> DQSDLHISDQTDTKGTVCSPFALFAVLENTGEKLKKSKWKWELHKLENARKPLKDGNVIEKG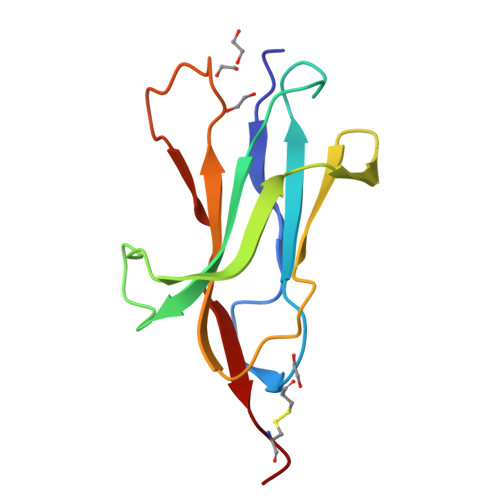FVSNQIGDSLYKIETKKKMKPGIYAFKVYKPAGYPANGSTFEWSEPMRLAKCDE> MGSSHHHHHSSGLVPRGSHMLSIKDLHVSVEDKAILRGLSLD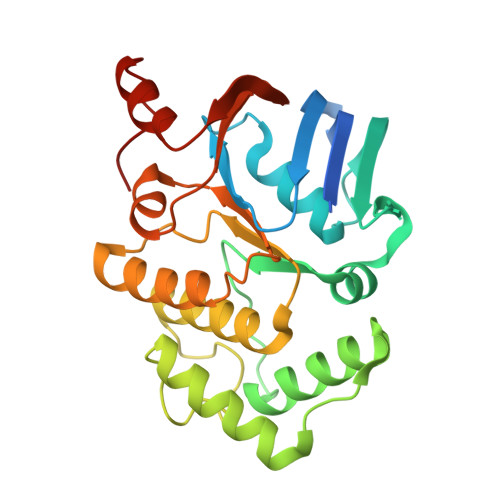VHPGEVHAIMGPNGSGKSTLSATLAGREDYEVTGGTVEFKGKDLLALSPEDRAGEGIFMAFQYPVEIPGVSNQFFLQTALNAVRSYRGQETLDRFDFQDLMEEKIALLKMPEDLLTRSVNVGFSGGEKKRNDILQMAVLEPELCILDESDSGLDIDALKVVADGVNSLRDGKRSFIIVTHYQRILDYIKPDYVHVLYQGRIVKSGDFTLVKQLEEQGYGWLTEQQ2-(1,4,5,6-tetrahydropyrimidin-2-yl)benzenethiol 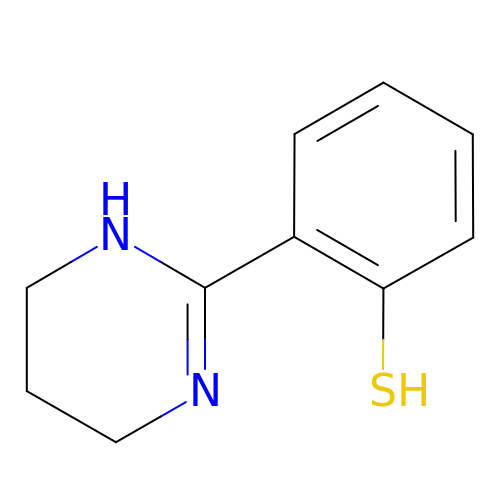| C10 H12 N2 S | DUHDUYRXLGSMLQ-UHFFFAOYSA-N2-[[(2R)-1-[[(2S)-5-amino-1-[(4-carbamimidoylphenyl)methylamino]-1,5-dioxo-pentan-2-yl]amino]-3-(1H-indol-3-yl)-1-oxo-propan-2-yl]sulfamoyl]ethanoic 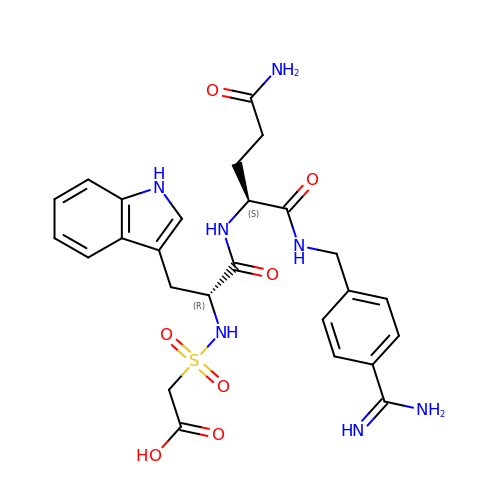acid | C26 H31 N7 O7 S | NLKRKTGGXZDTOO-LEWJYISDSA-N>[4x]AYVEIIEQPKQRGMRFRYKCEGRSAGSIPGERSTDTTKTHPTIKINGYTGPGTVRISLVTKDPPHRPHPHELVGKDCRDGYYEADLCPDRSIHSFQNLGIQCVKKRDLEQAISQRIQTNNNPFHVPIEEQRGDYDLNAVRLCFQVTVRDPAGRPLLLTPVLSH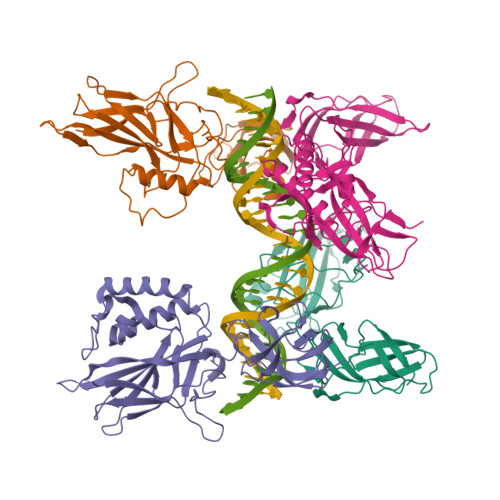PIFDNRAPNTAELKICRVNRNSGSCLGGDEIFLLCDKVQKEDIEVYFTGPGWEARGSFSQADVHRQVAIVFRTPPYADPSLQAPVRVSMQLRRPSDRELSEPMEFQYLPD;>GPYLQILEQPKQRGFRFRYVCEGPSHGGLPGASSEKNKKSYPQVKICNYVGPAKVIVQLVTNGKNIHLHAHSLVGKHCEDGVCTVTAGPKDMVVGFANLGILHVTKKKVFETLEARMTEACIRGYNPGLLVHSDLAYLQAEGGGDRQLTDREKEIIRQAAVQQTKEMDLSVVRLMFTAFLPDSTGSFTRRLEPVVSDAIYDSKAPNASNLKIVRMDRTAGCVTGGEEIYLLCDKVQKDDIQIRFYEEEENGGVWEGFGDFSPTDVHRQFAIVFKTPKYKDVNITKPASVFVQLRRKSDLETSEPKPFLYYPE[4x]> MQFSKMHGLGNDFVVVDGVTQNVFFTPETIRRLANRHCGIGFDQLLIVEAPYDPELDFHYRIFNADGSEVSQSGNGARCFARFVTLKGLTNKKDISVSTQ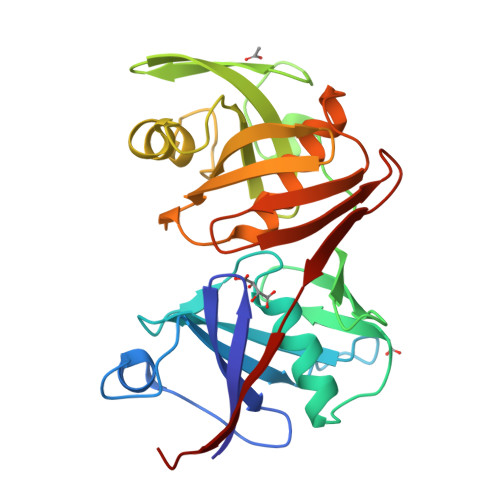KGNMVLTVKDDNQIRVNMGEPIWEPAKIPFTANKFEKNYILRTDIQTVLCGAVSMGNPHCVVQVDDIQTANVEQLGPLLESHERFPERVNAGFMQIINKEHIKLRVYERGAGETQACGSGACAAVAVGIMQGLLNNNVQVDLPGGSLMIEWNGVGHPLYMTGEATHIYDGFITL>MGSDKIHHHHHHTEGWFMPFDNWLYQLQNADPVEISSSGFEIAVIDYS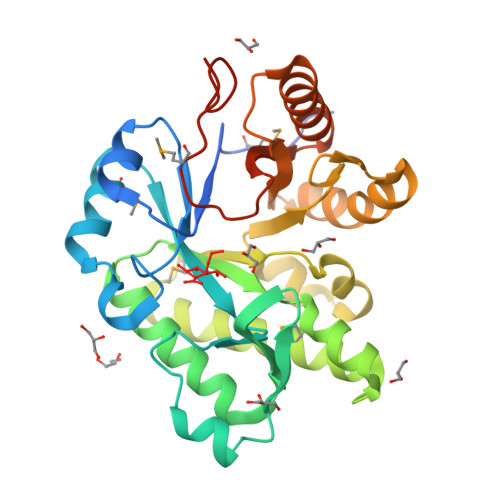KDGSESGEYSPEEIKIMVDAGVVPVAYVNIGQAEDYRFYWKESWYTNTPEWLGEEDPAWPGNYFVKYWYNEWKEIVFSYLDRVIDQGFKGIYLDRIDSFEYWAQEGVISRRSAARKMINFVLEIAEYVRERKPDMLIIPQNGENILDFDDGQLASTVSGWAVENLFYLKTIPLEENETKSRLEYLIRLNRKGKFILSVDYVDDGSDSFENISRILDYYEKAKRNGCIPYAARSDLELDEMNVIEGIQPPEALKDYESRTYR[6x]>[5x]MIVTTTSGIQGKEIIEYIDIVNGEAIMGANIVRDLFA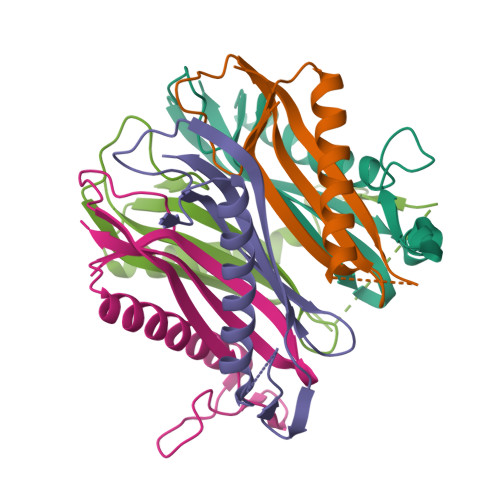SVRDVVGGRAGSYESKLKEARDIAMDEMKELAKQKGANAIVGVDVDYEVVRDGMLMVAVSGTAVRI3-({(2S)-2-[({(1R)-1-[({(1R)-1-[(R)-CARBOXY(HYDROXY)METHYL]-3,3-DIFLUOROPROPYL}AMINO)CARBONYL]-3-METHYLBUTYL}AMINO)CARBONYL]-2,3-DIHYDRO-1H-INDOL-2-YL}METHYL)THIOPHENE-2-CARBOXYLIC ACID | C26 H31 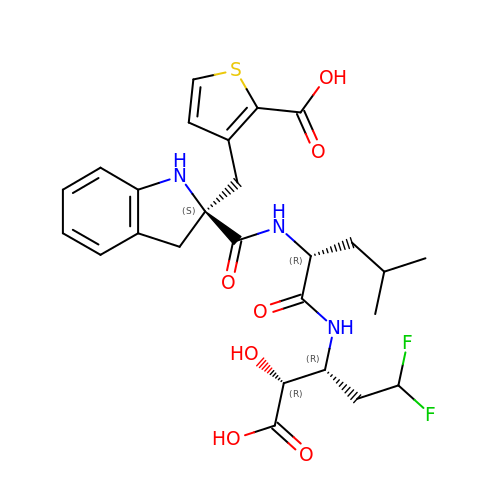F2 N3 O7 S | BEFPIHVRQQQFFB-DUFVWYDBSA-N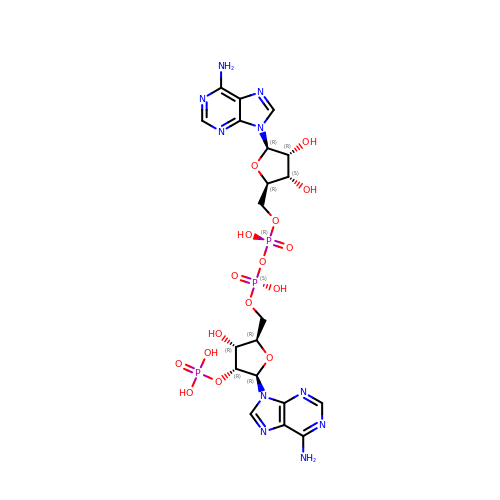[(2R,3S,4R,5R)-5-(6-AMINO-9H-PURIN-9-YL)-3,4-DIHYDROXYTETRAHYDROFURAN-2-YL]METHYL [(2R,3R,4R,5R)-5-(6-AMINO-9H-PURIN-9-YL)-3-HYDROXY-4-(PHOSPHONOOXY)TETRAHYDROFURAN-2-YL]METHYL DIHYDROGEN DIPHOSPHATE | C20 H27 N10 O16 P3 | JRSFRHPGKHPNEL-XPWFQUROSA-N N-(IMINOMETHYL)-L-GLUTAMIC ACID | C6 H10 N2 O4 | 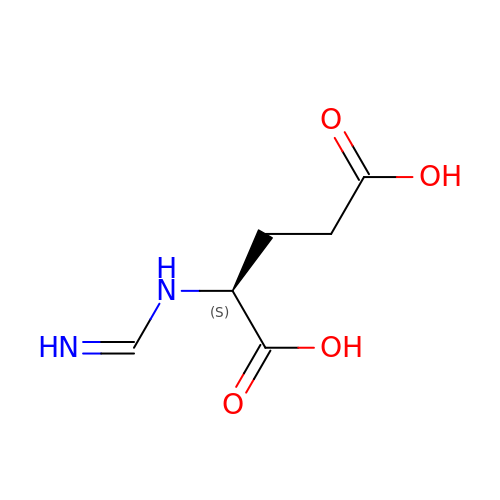NRXIKWMTVXPVEF-BYPYZUCNSA-N>[2x]SE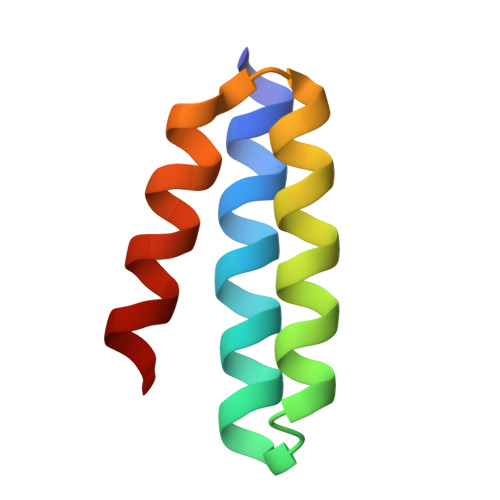ESEKLLKEAKEEVRRLFEEGRPEDAARVAFEFLQRLLDLGDPDAVKELLQFLRELL>[2x]MGKTDQQVGAKLVQEIREGKRGPLYAGYFRT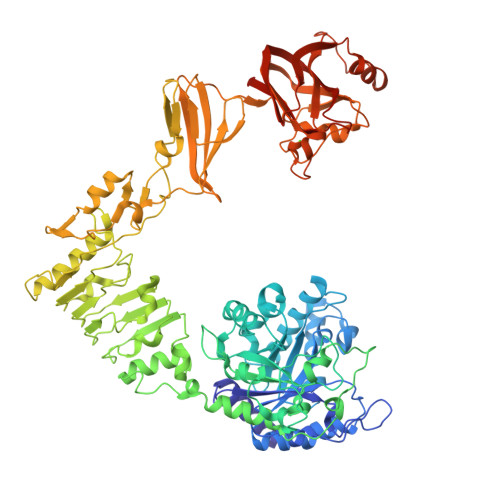WHDRASTGIDGKQQHPENTMAEVPKEVDILFVFHDHTASDSPFWSELKDSYVHKLHQQGTALVQTIGVNELNGRTGLSKDYPDTPEGNKALAAAIVKAFVTDRGVDGLDIDIEHEFTNKRTPEEDARALNVFKEIAQLIGKNGSDKSKLLIMDTTLSVENNPIFKGIAEDLDYLLRQYYGSQGGEAEVDTINSDWNQYQNYIDASQFMIGFSFFEESASKGNLWFDVNEYDPNNPEKGKDIEGTRAKKYAEWQPSTGGLKAGIFSYAIDRDGVAHVPSTYKNRTSTNLQRHEVDNISHTDYTVSRKLKTLMTEDKRYDVIDQKDIPDPALREQIIQQVGQYKGDLERYNKTLVLTGDKIQNLKGLEKLSKLQKLELRQLSNVKEITPELLPESMKKDAELVMVGMTGLEKLNLSGLNRQTLDGIDVNSITHLTSFDISHNSLDLSEKSEDRKLLMTLMEQVSNHQKITVKNTAFENQKPKGYYPQTYDTKEGHYDVDNAEHDILTDFVFGTVTKRNTFIGDEEAFAIYKEGAVDGRQYVSKDYTYEAFRKDYKGYKVHLTASNLGETVTSKVTATTDETYLVDVSDGEKVVHHMKLNIGSGAIMMENLAKGAKVIGTSGDFEQAKKIFDGEKSDRFFTWGQTNWIAFDLGEINLAKEWRLFNAETNTEIKTDSSLNVAKGRLQILKDTTIDLEKMDIKNRKEYLSNDENWTDVAQMDDAKAIFNSKLSNVLSRYWRFCVDGGASSYYPQYTELQILGQRLSNDVANTLKDL> ITQQQGATWGL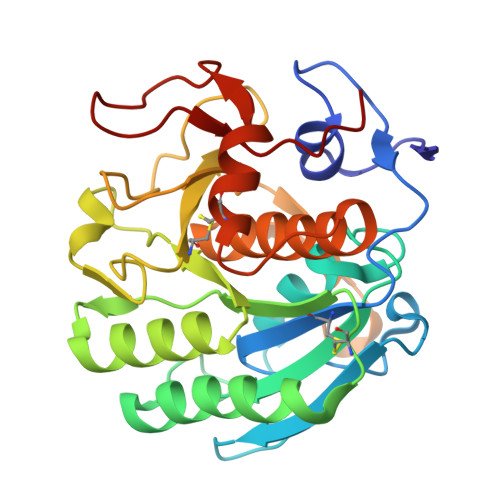TRISHRARGSTAYAYDTSAGAGACVYVIDTGVEDTHPDFEGRAKQIKSYASTARDGHGHGTHCAGTIGSKTWGVAKKVSIFGVKVLDDSGSGSLSNIIAGMDFVASDRQSRNCPRRTVASMSLGGGYSAALNQAAARLQSSGVFVAVAAGNDNRDAANTSPASEPTVCTVGATDSNDVRSTFSNYGRVVDIFAPGTSITSTWIGGRTNTISGTSMATPHIAGLAAYLFGLEGGSAGAMCGRIQTLSTKNVLTSIPSGTVNYLAFNGAT>MSLLPRTTSVKPGEKFDVIIVGLGPAAYGAALYSARYMLKTLVIGETPGGQLTEAGIVDDYLGLIEIQASDMIKVFNKHIEKYEVPVLLDIVEKIENRGDEFVVKTKRKGEFKADSVILGIGVKRRKLGVPGEQEFAGRGISYCSVCDAPLFKNRVVAVIGGGDSALEGAEILSSYSTKVYLIHRRDTFKAQPIYVETVKKKPNVEFVLNSVVKEIKGDKVVKQVVVENLKTGEIKELNVNGVFIEIGFDPPTDFAK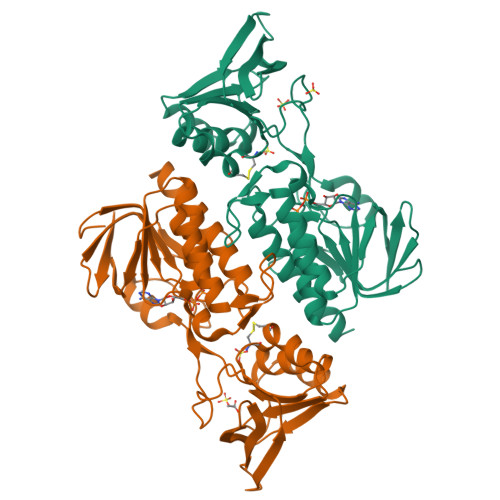SNGIETDTNGYIKVDEWMRTSVPGVFAAGDCTSAWLGFRQVITAVAQGAVAATSAYRYVTEKKGKK[4x]>[2x]TRDQNGTWEME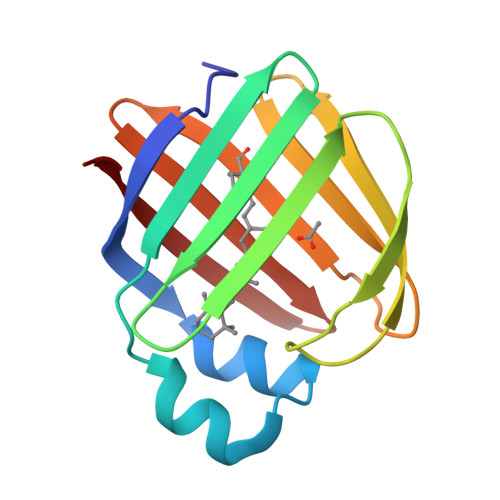SNENFEGWMKALDIDFATRKIAVRLTQTLVIDQDGDNFKVKTTSTFYNYDVDFTVGVEFDEYTKSLDNRHVKALVTWEGDVLVCVQKGEKENRGWKKWIEGDKLYLELTCGDQVCRQVFKKK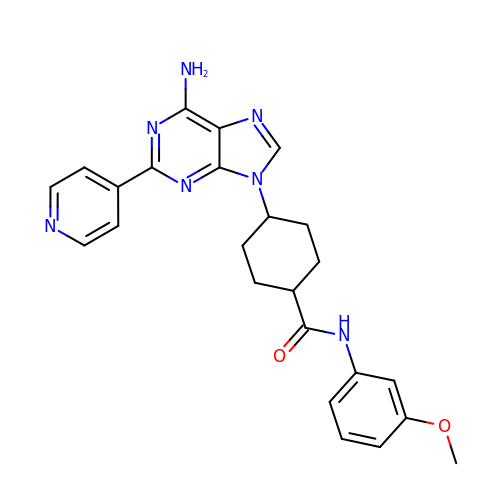4-(6-azanyl-2-pyridin-4-yl-purin-9-yl)-~{N}-(3-methoxyphenyl)cyclohexane-1-carboxamide | C24 H25 N7 O2 | JLJXNSYNQKBEKE-MAEOIBBWSA-N>[3x]NDKICAGVASGKGTHRVETITKGEVLVTNAINMTHTPTSGPFGDLKTGNVRDKLCPTCTGCTDMDVALMTPTCNGVIPEAIAAIQHENRPLQSKCNPILHDLGNTRQLPNLLRKYKKIRKSSGIAFPLASYADQPVISNPSGNCRDGNGVESEFGSLLWLTGNTKGAITGETITITHQCNNDEVMVLVWGAWADLSATMNTIYGVTTPQTYVSNFPSGRFSMSPFLGNFPALAETEATTATGRIYLRMEVLESGQRGTIQYQRGFMGPGKFWCLSEPIPVVKGAVKTNGAVSDCLHEVYGGISKPTPFYTGNRGKSVGNCPKWVRKPLLVVNGTKAR;>[3x]DSISTRGLFGAIAGFLEGGWDGMIAGWHGYSSTGDHGTKVAADLVSTQKAMDAITARINNMNKMTERAFSVTDSTMQEIQKEIKDLDKKIDDVRADETAAQIEMIVLLENEN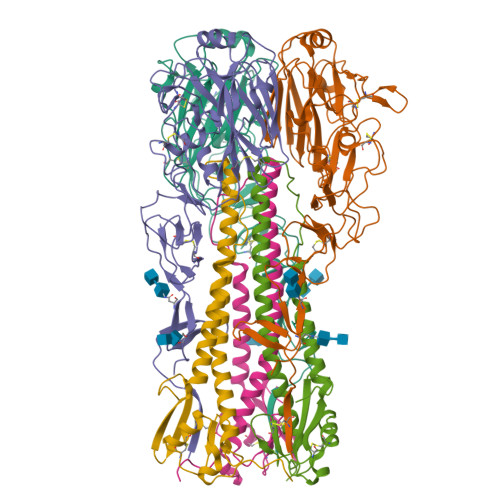IINAEDEHVHALKQKLTKMLGPSAQDMGDGCFIVDHQCKEDCLREIVSGNYTPSKYGMDEFKSPIITGT The broad substrate specificity and cellular functions of PP2A are controlled by formation of diverse heterotrimeric holoenzymes; each contains a common core enzyme formed by the scaffold (A) and catalytic (C or PP2Ac) subunits and a third variable regulatory subunit from four major families (B/B55/PR55, B’/B56/PR61, B”/PR72, and B”’/Striatin). TIPRL (target of rapamycin (TOR) signaling pathway regulator) is an important PP2A inhibitory protein and forms a complex with PP2Ac together with α431, excluding both scaffold and regulatory subunits. We determined the crystal structures of mouse TIPRL and its complex with the PP2A core enzyme at 2.7 and 3.8 Å, respectively. Structure-guided studies reveal that TIPRL inhibits PP2A by perturbing the phosphatase active site, and together with α4, exhibits a robust activity in disassembly of active PP2A holoenzymes in a highly sensitive methylation-responsive manner.

TIPRL possesses a unique butterfly-shaped protein fold with two extended layers of β-sheets that pack closely and in parallel at the center. Several helical wings (HWs) arch outward to give an overall butterfly-shaped structure. TIPRL structure is very similar between mouse and human 35 and is likely conserved across species due to a high level of sequence similarity.

> GSDFSFGPWKLTASKTHIMKSADVEKLADELHMPSLPEMMFGDNVLRIQHGSGFGIEFNATDALRCVNNYQGMLKVACAEEWQEVIKPYDWTYTTDYKGTLLGESLKLKVVPTTDHIDTEKLKAREQIKFFEEVLLFEDELHDHGVSSLSVKIRVMPSSFFLLLRFFLRIDGVLIRMNDTRLYHEADKTYMLREYTSRESKIANLMHVPPSLFTEPNEISQYLPIKEAVCEKLVFPERID>MAKRKIQRYVRKDGKCNVHHGNVRETYRYLTDIFTTLVDLKWRFNLLIFVMVYTVTWLFFGMIWWLIAYIRGDMDHIEDPSWTPCVTNLNGFVSAFLFSIETETTIGYGYRVITDKCPEGIILLLIQSVLGSIVNAFMVGCMFVKISQPKKRAETLVFSTHAVISMRDGKLCLMFRVGDLRNSHIVEASIRAKLIKSKQTSEGEFIPLNQTDINVGYYTGDDRLFLVSPLIISHEINQQSPFWEISKAQLPKEELEIVVILEGMVEATGMTCQARSSYITSEILWGYRFTPVLTLEDGFYEVDYNSFHET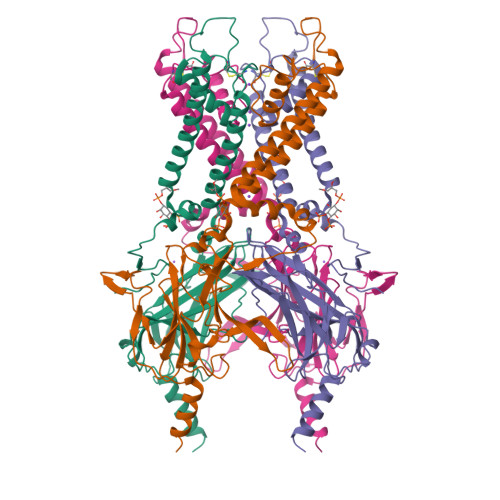YETSTPSLSAKELAELANRAESNSLEVLFQ[4x]>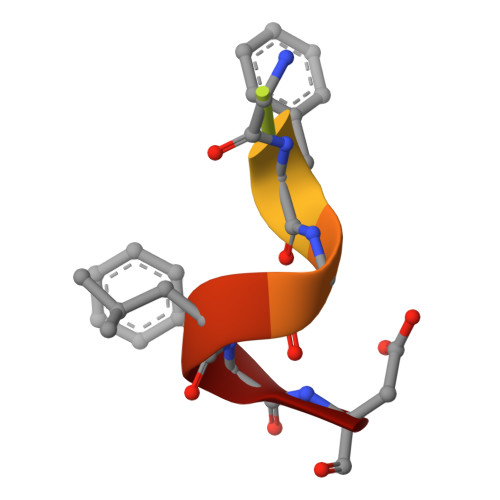 DDDMGFGLFD1-[(2S)-2-(3-methoxyphenyl)pyrrolidin-1-yl]ethan-1-one | C13 H17 N O2 | 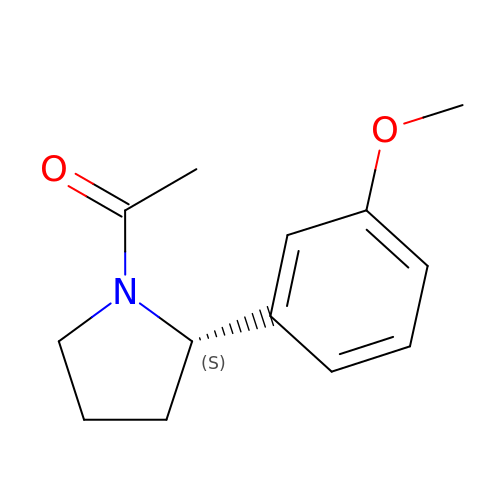BTTYWNVACUVDJT-ZDUSSCGKSA-N> FARLKRSLLKTKENLGSGFISLFRGKKIDDDLFEELEEQLLIADVGVETTRKIITNLTEGASRKQLRDAEALYGLLKEEMGEILAKVDEPLNVEGKAPFVILMVGVNGVGKTTTIGKLARQFEQQGKSVMLAA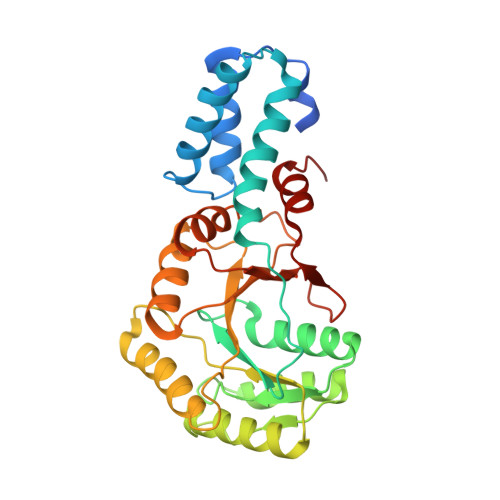GDTFRAAAVEQLQVWGQRNNIPVIAQHTGADSASVIFDAIQAAKARNIDVLIADTAGRLQNKSHLMEELKKIVRVMKKLDVEAPHEVMLTIDASTGQNAVSQAKLFHEAVGLTGITLTKLDGTAKGGVIFSVADQFGIPIRYIGVGERIEDLRPFKADDFIEALFARED> ATLKDITRRLKSIKNIQKITKSMKMVAAAKYARAERELKPARVYGTGSLALYEKAEIKGPEDKKKHLIIGVSSDRGLCGAIHSSVAKQMKNDMAALTAAGKEVMIVGIGEKIKSIL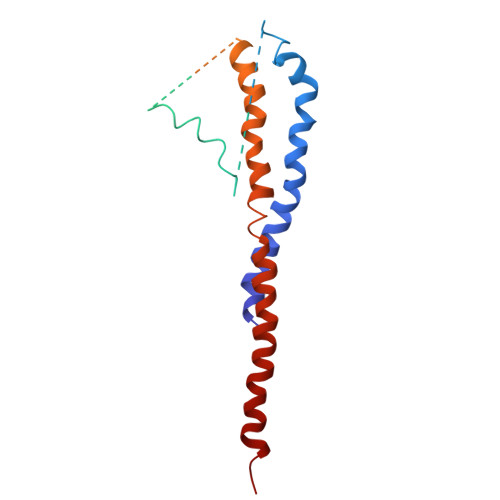YRTHSDQFLVSFKDVGRKPPTFGDASVIALELLNSGYEFDEGSIIFNQFKSVISYKTEEKPIFSFSTVVAAENMSIYDDIDADVLQNYQEYNLANIIYYSLKESTTSEQSARMTAMDNASKNASDMIDKLTLTFNRTRQAVITKELIEIISGAAALD> SLFYNPQKMLSYDRILNFVIGARGIGKSYAMKVYPINRFIKYGEQFIYVRRYKPELAKVSNYFNDVAQEFPDHELVVKGRRFYIDGKLAGWAIPLSVWQSEKSNAYPNVSTIVFDEFIREKDNSNYIPNEVSALLNLMDTVFRNRERVRCICLSNAVSVVN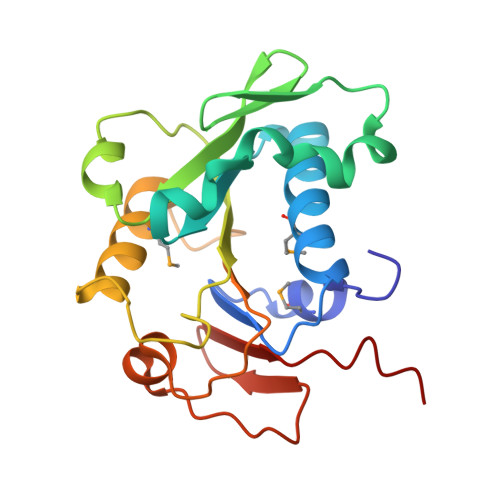PYFLFFNLVPDVNKRFNVYDDALIEIPDSLDFS>SNAMKTIRTQTPLRLGLAGGGTDINLYCDKYTGYVLNATISLYIHCTLIKREDGKIIFDSPDTNSYCEYESKEFLGNDGKLDIFKSIYNRIVKDFTKKPLSFSLHTYSDVPSGSGLGGSSTLVVGVIKAFAEWLNLPLGEYEIAKLAYEIEREDLGIVGGAQDQYAATFGGFNFMEFYNNKRVIVNPLRIKNWIASELEARTVLYFTNITREAKDIEEHKKGK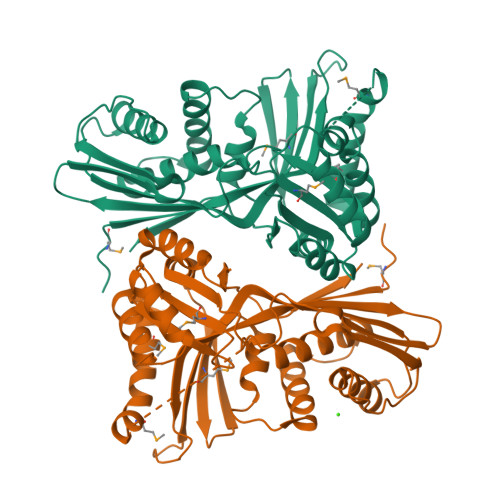LGDEKSLEAMHAIKQDAIKMKEALFRADFGTLAQILGKSWRSKKIISEIVSNDELERIYKLAIDNGAYSGKTSGAGAGGFMFFFVDPTKKYNLIKALRKEQGYVQDFSFTKEGVKSWRI[2x]Human SNM1B (SNM1B, Apollo, or DCLRE1B) is a 5′-to-3′ exonuclease, which was first identified as one of three vertebrate orthologues of the yeast DNA repair nuclease, PSO2 (4). SNM1B is a member of the metallo-β-lactamase (MBL) structural superfamily, of which the β-CASP (CPSF, Artemis, SNM1, PSO2) nucleic acid processing nucleases are a subfamily. All MBL type enzymes possess a characteristic α/β/β/α MBL core fold that provides a scaffold that supports the active site, which coordinates the metal ions essential for catalysis. The SNM1B sequence comprises 532 amino acids, wherein the N-terminal region (amino acids 1–332) contains the catalytic (MBL and β-CASP) domains, and the C-terminal region the protein-protein interaction regions, including the well-characterised TRF2 binding domain (amino acids 498–509).

An SNM1B coding variant, H61Y, correlates with an increased risk of breast cancer. This substitution is in the MBL domain, being located adjacent to the active site. We solved a structure of H61Y SNM1B1–355 (3.2 Å resolution). The overall architecture of this is extremely similar to WT with a backbone root mean squared deviation (RMSD) of 0.3 Å (312 residues to 312 residues). The structure around the active site is also near identical. There is only minor perturbation of the Y61 neighbouring residues (R60, Q63, R206, R207 and E209), and no effect to the α-helix that Y61 resides in, or the adjacent helix, which contains many of the nearby residues. WT and H61Y SNM1B1–355 showed similar thermal denaturation profiles, suggesting that the H61Y variant does not substantially perturb its fold. The H61Y Michaelis-Menten kinetics, as measured by a real-time fluorescence-based nuclease activity were comparable to WT, as was its ability to bind ssDNA in the FP binding assay. Our study on the structure, and properties, of the breast cancer associated, H61Y variant of SNM1B1–355 reveal its fold is very similar to unliganded WT SNM1B1–355 and appears equivalent to WT SNM1B1–355 with regards to thermal stability, DNA binding, catalytic efficiency, and nuclease activity. Thus, it would seem likely that the reported deleterious associations of rs11552449 and cancer risk may be mediated by the effects of alternative transcript splicing, rather than the non-synonymous substitution in the protein-coding sequence.

> SMGYGNGVLIPHTPIAVDFWSLRRAGTARLFFLSHMHSDHTVGLSSTWARPLYCSPITAHLLHRYLQVSKQWIQALEVGESHVLPLDEIGQETMTVTLLDANHCPGSVMFLFEGYFGTILYTGDFRYTPSMLKEPALTLGKQIHTLYLDNTNCNPALVLPSRQEAAHQIVQLIRKHPQHNIKIGLYSLGKESLLEQLALEFQTWVVLSPRRLELVQLLGLADVFTVEEKAGRIHAVDHMEICHSNMLRWNQTHPTIAILPTSRKIHSSHPDIHVIPYSDHSSYSELRAFVAALKPCQVVPIVSRRPCGGFQDSLSPRISVPLIPDSVQQYMSSSSRKPS>SNAMASLHIDDIPAAIKAVKQQLRQALPDYQQVFQAVEENIRQQVMEIRRNLAEGKNPVPQLHADDIINGKVTEEQKAQIKQRGCCAILGVFPQEKATAWNREIGDYLDRNNFVERLKNAAEDNYFGTLAASKPQIYGIYWSTPQVEARQDKRMQAVQIFLNNLWQTESNGKQHFDANRVVTYADRTRRRPPKSSSLGLSPHVDGGSIERWLDENFRHVYRHVFSGQWQKYDPFAAEGRPEVREFPSPAVCSMFRTFQGWTALTPQRTHAGTLNVIPIANAMAYILLRALQDDVADDDLCGAAPGRALSASEQWHPLLMEAISPIPDLEAGDTVFWHCDVIHSVENEHNGEFD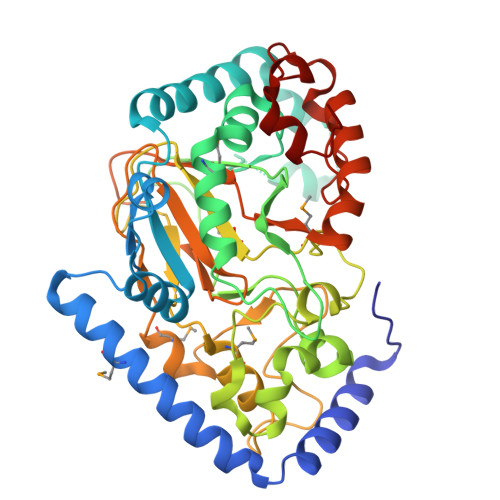SNVMYIAAAPWCEKNAAYLPRQLASFIDGRSPPDFAADDFEVDFIGRATIKNLTEIGKQQLGITD[2x]(2Z,6E)-2-fluoro-3,7,11-trimethyldodeca-2,6,10-trien-1-yl trihydrogen diphosphate | C15 H27 F O7 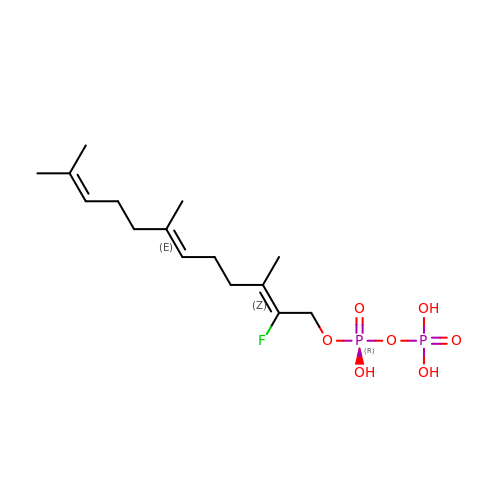P2 | DXHJZCKJWKWTCH-WISUYLHISA-N> AERPTLPIPDLLTTDARNRIQLTIGAGQSTFGGKTATTWGYNGNLLGPAVKLQRGKAVTVDIYNQLTEETTLHWHGLEVPGEVDGGPQGIIPPGGKRSVTLNVDQPA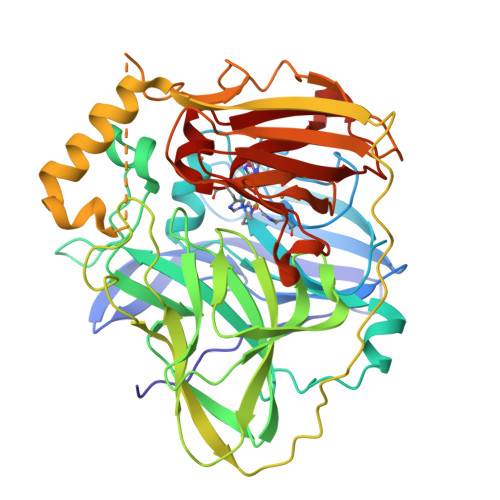ATCWFHPHQHGKTGRQVAMGLAGLVVIEDDEILKLMLPKQWGIDDVPVIVQDKKFSADGQIDYQLDVMTAAVGWFGDTLLTNGAIYPQHAAPRGWLRLRLLNGCNARSLNFATSDNRPLYVIASDGGLLPEPVKVSELPVLMGERFEVLVEVNDNKPFDLVTLPVSQMGMAIAPFDKPHPVMRIQPIAISASGALPDTLSSLPALPSLEGLTVRKLQLSMDPMLDMMGMQMLMEKYGDQAMAGMDHSQMMGHMGHGNMNHMNHGGKFDFHHANKINGQAFDMNKPMFAAAKGQYERWVISGVGDMMLHPFHIHGTQFRILSENGKPPAAHRAGWKDTVKVEGNVSEVLVKFNHDAPKEHAYMAHCHLLEHEDTGMMLGFTV> MTHAELHLFDLDEFMQTYKRLQTRQDWLIENKCKKSRLFSYVAAVIAFTVGKSATMSDEAILAKIDPYVTSEVRVQRGAWWRSGYFTKEEVEMMTPKGPIARYYKFLLGVR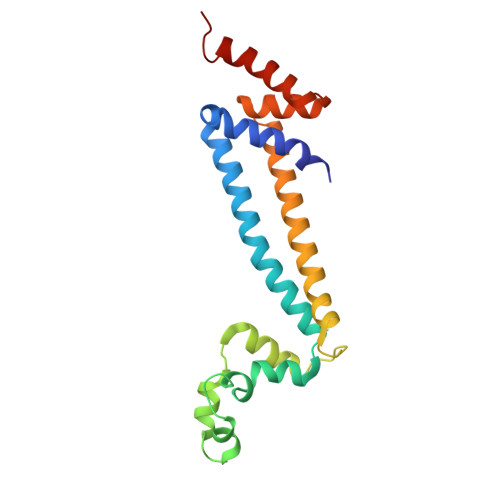RFPLKHGALSWACGFVPAWLTFTSLNHWAQNRRLNRYLTQESVFGEMARELVRGKTADEATTSVMARVEKEILGVH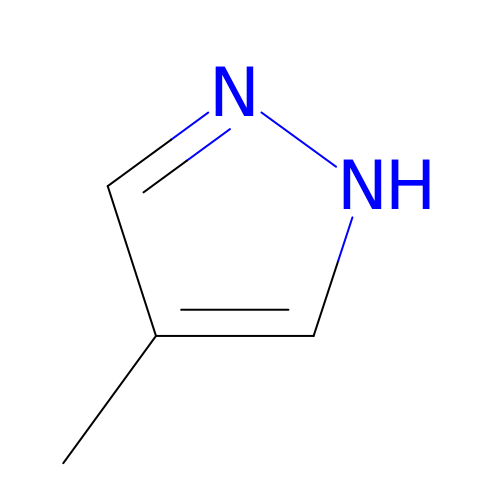4-methyl-1H-pyrazole | C4 H6 N2 | RIKMMFOAQPJVMX-UHFFFAOYSA-N>[2x]MKKKIGLLVMAYGTPYKEEDIERYYTHIRRGRKPSPEMLEDLTERYRAIGGISPLATITLEQAKKLEKRLNEVQDEVEYHMYLGLKHIEPFIEDAVKEMHNDGIQDAIALVLAPHYSTFSVKSYVGRAQEEAEKLGNLTIHGIDSWYKEPKFIQYWVDAVKSIYSGMSDAEREKAVLIVSAHSLPEKIIAMGDPYPDQLNETADYIARGAEVANYAVGWQSAGNTPDPWIGPDVQDLTRELNEKYGYT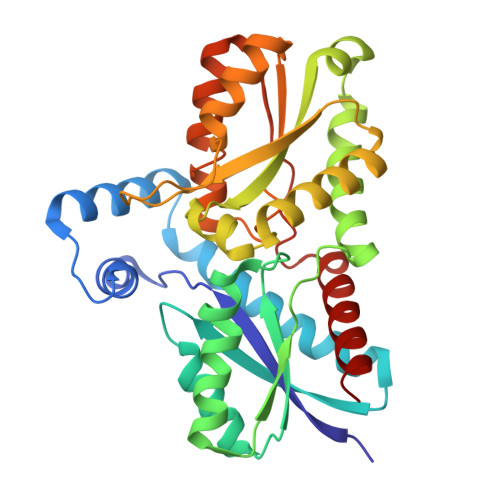SFVYAPVGFVAEHLEVLYDNDFECKVVTDEIGAKYYRPEMPNASDAFIDCLTDVVVKKKESVM2-methyl-5-propan-2-yl-phenol 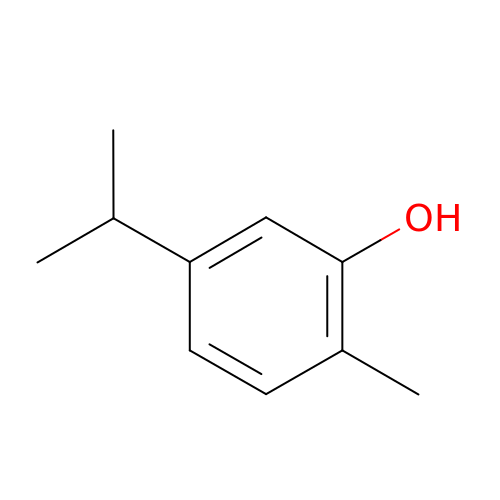| C10 H14 O | RECUKUPTGUEGMW-UHFFFAOYSA-N octyl 4-O-beta-D-allopyranosyl-1-thio-beta-D-altropyranoside 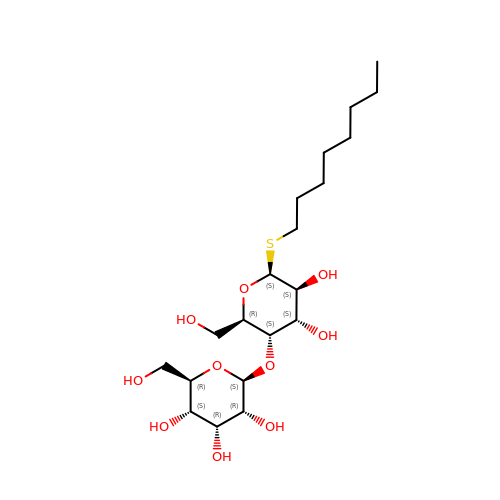| C20 H38 O10 S | JHBBNAKIOKQRJS-AIIAIXEESA-N>[2x]TAQTQTHLNFTQIKTVDELNQALVEAKGKPV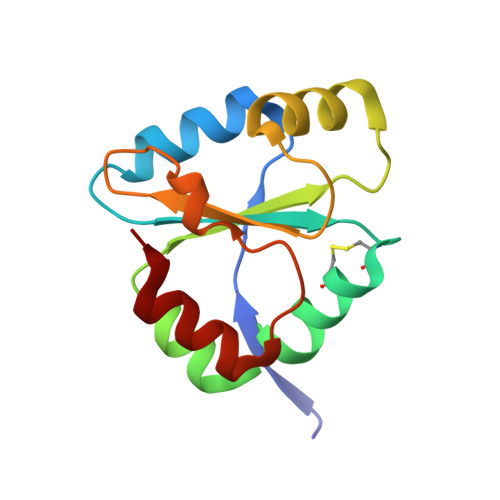MLDLYADWCVACKEFEKYTFSDPQVQKALADTVLLQANVTANDAQDVALLKHLNVLGLPTILFFDGQGQEHPQARVTGFMDAETFSAHLRDRQP>[4x]GPHMAAAAMAAAAGGGAGAARSLSRFR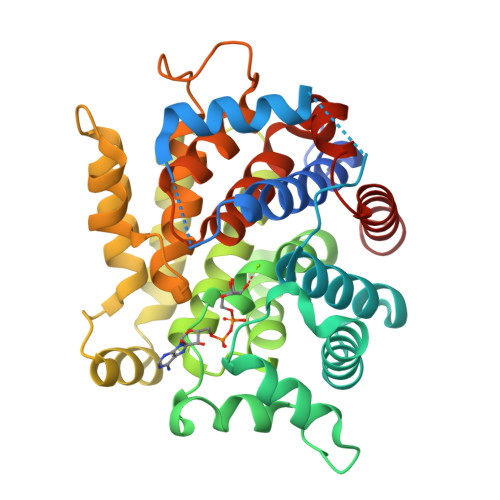GCLAGALLGDCVGSFYEAHDTVDLTSVLRHVQSLEPDPGTPGSERTEALYYTDDTAMARALVQSLLAKEAFDEVDMAHRFAQEYKKDPDRGYGAGVVTVFKKLLNPKCRDVFEPARAQFNGKGSYGNGGAMRVAGISLAYSSVQDVQKFARLSAQLTHASSLGYNGAILQALAVHLALQGESSSEHFLKQLLGHMEDLEGDAQSVLDARELGMEERPYSSRLKKIGELLDQASVTREEVVSELGNGIAAFESVPTAIYCFLRCMEPDPEIPSAFNSLQRTLIYSISLGGATDTIATMAGAIAGAYYGMDQVPESWQQSCEGYEETDILAQSLHRVFQKS>MTSLSGVTLNDACVETYQQLKLGKKLKYIIFHLNKENTEIAVEKSSDSVDYDNF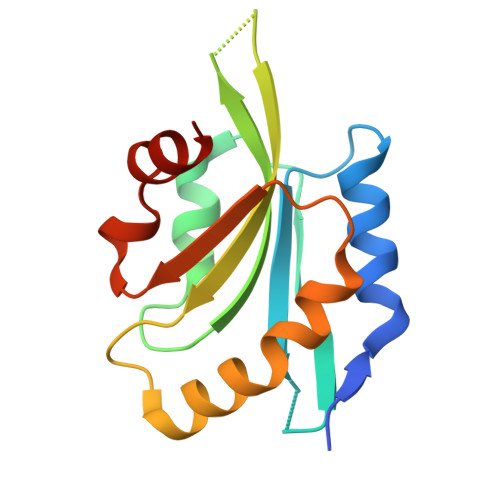LADLPEDECRWAVYDLEYEKEEGAGKRNKLTFVSWAPDSAKMKQKMAYASSKDILRRALTGIAVEIQGTDFSEVAHENVLDKASRGH[2x]Crocagins (1 and 2)24 are very small, intriguing RiPPs that possess a tetracyclic ring system, which consists of a pyrroloindoline fused to a tetrahydropyrimidinone moiety. Here we use in vitro experiments to demonstrate that three proteins, CgnB, CgnC and CgnE, are sufficient for the production of the hallmark tetracyclic crocagin core from the precursor peptide CgnA. We further show that the hydrolase CgnD liberates the crocagin core scaffold, which is subsequently N-methylated by CgnL. The crystal structures of the homologues CgnB and CgnE reveal them to be the founding members of a peptide-binding protein family and allow us to rationalize their distinct functions.

CgnB was recalcitrant to crystallization until a slight molar excess of CgnA was added prior to crystallization trials. We determined the CgnB structure to 2.3 Å resolution but observed no electron density for CgnA, so the peptide may simply have acted as an additive to promote crystallization. Curiously, CgnB contained a dinuclear metal centre that was partially occupied. The binding sites comprised CgnB residues Glu161, Glu252 (shared between Zn2+ 1 and 2), Glu274 and His280 (Zn2+ 1) and His291 and Asp293 (Zn2+ 2). As expected for homologous proteins, the Cα root-mean-square deviation (r.m.s.d.) between the structures of CgnB and CgnE was only 1.2 Å over 284 residues. The aminopeptidases form an extensive dimer interface, and the residues involved in its formation are largely missing in CgnB and CgnE, which rationalizes their monomeric state in the crystals. The leader peptide is enriched with positively charged amino acids, and both CgnB and CgnE show a large, strongly negatively charged patch near the possible binding site. Hydroxylation at the Tyr20 Cβ position allows CgnB to catalyse an elimination reaction via its bound Zn2+ (or Co2+) ions, which results in a double bond between the Tyr20 Cα and Cβ atoms, creating a conjugated amine. The CgnE homologue CgnB on the other hand appears to possess catalytic activity.

>[2x]GAMADIGSMDVLEYFERLKNRELAFVLDDLQLSDMVTRRGFSVIPFDDFDLAREDHPPAFVLVTRLDYHGKLMQAWETAKGISSHLSLAKFDTSPKSVEYSLDQLLSMDFAETLKRRGDYYDSVASTNRMEVVTPGAVLTCDFGNEIEIANNDVEMQKGWLYSVAEFFETSVINLEADRSSYTLNGDLCFTGLIYLCNRPDLKERASATMDELMRMSTRGRNVVSFVDNQIVRMELGGVDMTATLRELIVGKEREGSSTEFAMGCVEYPLAQDWTINSVMNEGSHGIHVGVGMGKEIPHMDFIAKGAELRIAESSDA> KHK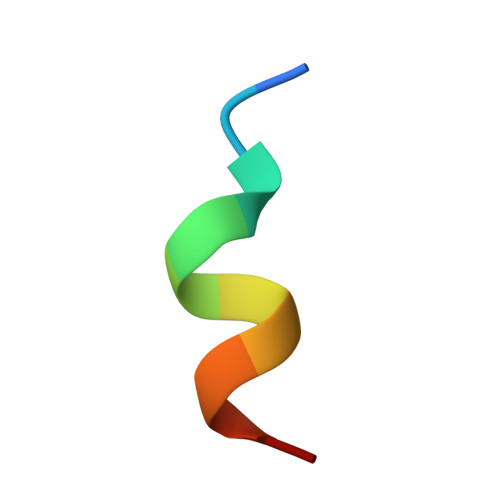ILHRLLQD> GPLGSMPNFSGNWKIIRSENFEELLKVLGVNVMLDDIAVAAASKPAVEIKQEGDTFYIKTSTTVRTTEINFKVGEEFEEQTVDGRPCKSLVKWESENKMVCEQKLLKGEGPKTSWTRELTNDGELILTMTADDV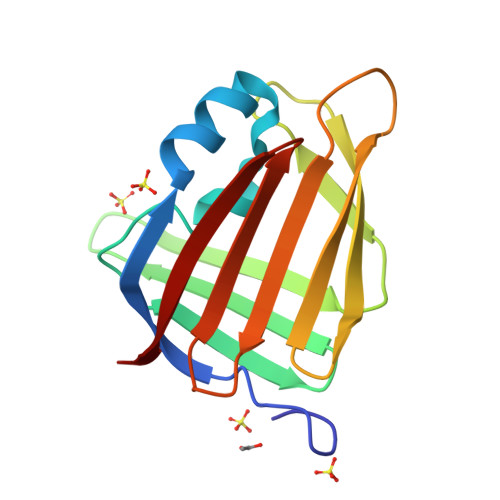VCTRVYVRE With the exception of α-hemolysin, which is homo-heptameric, leukotoxins are bipartite toxins, formed by the non-covalent association of two distinct proteins, a class S and a class F component of approximately 31 and 34 kDa, respectively, into a likely octameric species. Panton-Valentine leukocidin (PVL) is associated with necrotizing skin infections, such as boils, and plays an important role in the poor prognosis of necrotizing pneumonia. Two additional structural domains are also found: the rim domain anchors the protein to the membrane surface, while the stem domain, closely apposed to the core β-sandwich in the soluble form, contributes two β-strands to the pore β-barrel. Since the binding of LukS-PV to the membrane is a saturable process, the necessary presence of a LukS-PV receptor on the cell surface was thus proposed. This was recently confirmed by Spaan et al. who showed that the C5a receptor is required for the binding of LukS-PV to human neutrophils.

The mutants exhibiting significantly decreased binding abilities with respect to wild-type LukS-PV were: R73A, Y184A, T244A, H245A, and Y250A, with Ki values ranging from 1.8 to 6.2 nM, i.e. a 69- to 238-fold increase compared to the Ki value of wild-type LukS-PV. Four LukS-PV mutants (R73A, Y184A, T244A, and Y250) displayed significant alterations for all measured parameters, i.e. at least 50-fold decrease in affinity for hPMN membranes, 2-fold decrease in the slope of Ca2+ influx and 2- to 10-fold reduction in pore-forming capacity. The T244A, Y246A and N248A mutated proteins crystallized in identical conditions (50% PEG 200, 0.1 M MES-NaOH, pH 7.50). The corresponding crystals belonged to the P43212 space group, with similar cell parameters (a = b∼94 Å and c∼308 Å) and 4 molecules per asymmetric unit. These crystals diffracted X-rays at medium resolution (2.50 to 2.80 Å). In the case of the rim domain, wild-type LukS-PV and mutants T244A, Y246A and N248A displayed only small differences, with r.m.s. deviations comprised between 0.20 Å and 0.30 Å, whereas the structure of the rim domain of the Y184A and Y250A mutants were markedly different, with r.m.s. deviations of 1.10 Å and 1.28 Å, respectively, when compared to the wild-type LukS-PV structure. Three of the four most sensitive residues (Y184, T244 and Y250) are found in this region, at close distance from each other. Indeed, three of the five most sensitive residues identified (T244, H245 and Y250) are located in this loop and form a surface that could represent the principal binding site for the receptor.

>[4x]GPLGSPEFDNNIENIGDGAEVVKRTEDTSSDKWGVTQNIQFDFVKDKKYNKDALILKMQGFINSKTTYYNYKNTDHIKAMRWPFQYNIGLKTNDPNVDLINYLPKNKIDSVNVSQTLGYNIGGNFNSGPSTGGNGSFNYSKTISYNQQNYISEVEHQNSKSVQWGIKANSFITSLGKMSGHDPNLFVGYKPYSQNPRDYFVPDNELPPLVHSGFNPSFIATVSHEKGSGDTSEFEITYGRNMDVTHATRRTAHYGNSYLEGSRIHNAFVNRNYTVKYEVNWKTHEIKVKGHN> GPLGSMSEEQVAQDTEEVFRSYVFYRHQQEQEAEGVAAPADPEMVTLPLQPSSTMGQVGRQLAIIGDDINRRYDSEFQTMLQHLQPTAENAYEYFTKIATSLFESGINWGRVVALLGFGYRLALHVYQHGLTGFLGQVTRFVVDFMLHHSIARWIAQRGGW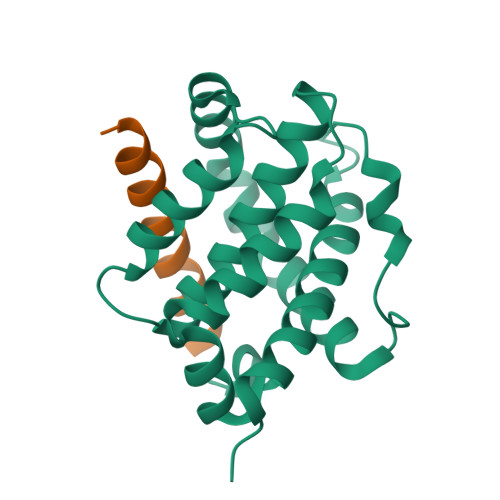VAALNLGNG;> XSYIDKIADLIRKVAEEINSKLEX> GSYPWILNHDHSKQKEISDWLTFEIKDFVAYISPSREEIEIRNQTISTIREAVKQLWPDADLHVFGSYST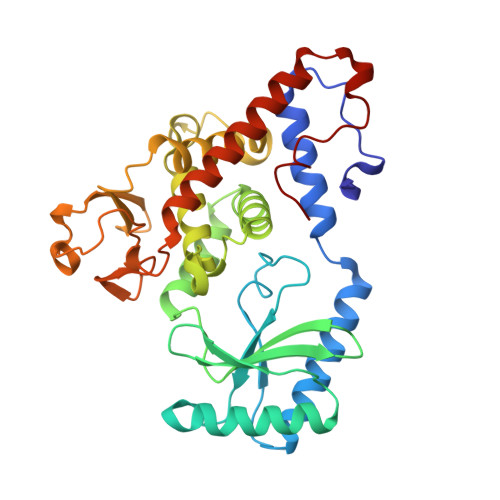DLYLPGSDIDCVVTSELGGKESRNNLYSLASHLKKKNLATEVEVVAKARVPIIKFVEPHSGIHIAVSFERTNGIEAAKLIREWLDDTPGLRELVLIVKQFLHARRLNNVHTGGLGGFSIICLVFSFLHMHPRIITNEIDPKDNLGVLLIEFFELYGKNFGYDDVALGSSDGYPVYFPKSTWSAIQPIKNPFSLAIQDPGDESNNISRGSFNIRDIKKAFAGAFDLLTNRCFELHSATFKDRLGKSILGNVIKY> METQLQSIFEEVVKTEIIEEAFPGMFMDTPEDEKTKLISCLAAFRQFWSGLSQESHEQCVQWIVKFIHGQHSPKRISFLYDCLAMAVETGLLPPRMVCESLINSDSLEWERTQLWALTFKLVRKIIGGVDYKGVRDLLKAILEKILTIPNTVSSAVVQQLLAAREVIAYILERNACLLPAYFAVTEIRKLYPEGKLPHWLLGNLVSDFVDTFRPTARINSICGRCSLLPVVNNSGAICNSWKLDPATLRFPLKGLLPYDKDLFEPQTALLRYVLEQPYSRDMVCNMLGLNKQHKQRCPVLEDQLVDLVVYAMERSETEEKFDDGGTSQLLWQHLSSQLIFFVLFQFASFPHMVLSLHQKLAGRGLIKGRDHLMWVLLQFISGSIQKNALADFLPVMKLFDLLYPEKECIPVPDINKPQSTHAFAMTCIWIHLNRKAQNGDSTLQIPIPHSLKLHHEFLQQSLRNKSLQMNDYKIALLCNAYSTNSECFTLPMGALVETIYGNGIMRVPLPGTSCLASASVTPLPMNLLDSLTVHAKMSLIHSIATRVIKLAHTKSSVALAPALVETYSRLLVYMEIESLGIKGFISQLLPTVFKSHAWGILHTLLEMFSHRMHHIQPHYRVQLLSHLHTLAAVAQTNQNQLHLCVESTALRLITALGSSEVQPQFTRFLNDPKTVLSAESEELNRALILTLARATHVTDFFTGSDSIQGTWCKDILQTIMNFTPHNWASHTLSCFPAPLQAFFKQNNVPQESRFNLKKNVEEEYRKWKSMTDENEIITQFSVQGFPPLFLCLLWKMLLETDHISQIGYKVLERIGARALVAHVRTFADFLVYEFSTSAGGQQLNKCIEILNDMVWKYNIVTLDRLILCLAMRSHEGNEAQVCYFIIQLLLLKPNDFRNRVSDFVKENSPEHWLQSDWHTKHMSYHKKYPEKLYFEGLAEQVDPPVPIQSPYLPIYFGNVCLRFLPVFDIVIHRFLELLPVSKSLETLLDHLGGLYKFHDRPVTYLYNTLHYYEMCLRNRDHLKRKLVHAIIGSLKDNRPQGWCLSDTYLKHAMNAREDNPWVPEDSYYCKLIGRLVDTMAGKSPGPFPNCD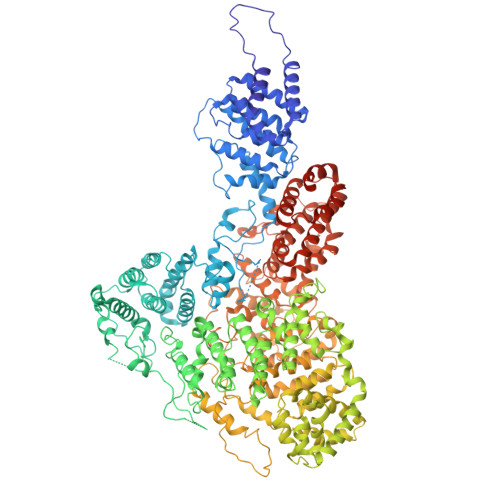WRFNEFPNPAAHALHVTCVELMALAVPGKDVGNALLNVVLKSQPLVPRENITAWMNAIGLIITALPEPYWIVLHDRIVNVISSSSLTSETEWVGYPFRLFDFTACHQSYSEMSCSYTLALAHAVWHHSSIGQLSLIPKFLTEALLPVVKTEFQLLYVYHLVGPFLQRFQQERTRCMIEIGVAFYDMLLNVDQCSTHLNYMDPICDFLYHMKYMFTGDSVKEQVEKIICNLKPALKLRLRFITHISKMEPAVPPQALNSGSPAPQSNQVPASLPVTQ>KCETIHVAIVCAGYNASRDVVTLVKSVLFHRRNPLHFHLIADSIAEQILATLFQTWMVPAVRVDFYNADELKSEVSWIPNKHYSGIYGLMKLVLTKTLPANLERVIVLDTDITFATDIAELWAVFHKFKGQQVLGLVENQSDWYLGNLWKNHRPWPALGRGYNTGVILLLLDKLRKMKWEQMWRLTAERELMGMLSTSLADQDIFNAVIKQNPFLVYQLPCFWNVQLSDHTRSEQCYRDVSDLKVIHWNSPKKLRVKNKHVEFFRNLYLTFLEYDGNLLRRELFGCPSEADVNSENLQKQLSELDEDDLCYEFRRERFTVHRTHLYFLHYEYEPAADSTDVTLVAQLSMDRLQMLEAICKHWEGPISLALYLSDAEAQQFLRYAQGSEVLMSRHNVGYHIVYKEGQFYPVNLLRNVAMKHISTPYMFLSDIDFLPMYGLYEYLRKSVIQLDLANTKKAMIVPAFETLRYRLSFPKSKAELLSMLDMGTLFTFRYHVWTKGHAPTNFAKWRTATTPYRVEWEADFEPYVVVRRDCPEYDRRFVGFGWNKVAHIMELDVQEYEFIVLPNAYMIHMPHAPSFDITKFRSNKQYRICLKTLKEEFQQDMSRRYGFAALKYLTA[2x]

Like-acetylglucosaminyltransferase 1 (LARGE1) is a bifunctional glycosyltransferase (GTase) that plays a critical role in maintaining proper muscle function. This enzyme is responsible for a post-translational modification on the extracellular matrix receptor, α-dystroglycan (α-DG), which enables it to interact with proteins containing a laminin-G domain. The polysaccharide which LARGE1 synthesizes, termed matriglycan, is composed of xylose (Xyl) and glucuronic acid (GlcA) subunits in a linear repeating structure of [-3GlcA-β1,3-Xyl-α1-]n. LARGE1 is present in the Golgi as a type II membrane protein, composed of a transmembrane/cytosolic region, a predicted coiled-coil/stem (CC), and domains with xylosyltransferase (Xyl-T) and glucuronyltransferase (GlcA-T) catalytic activities, which are separated by a linker.

While obtaining the single-particle EM data, we also managed to crystallize the LARGE1ΔCC and to collect X-ray diffraction data, extending to 2.6 Å. The crystal of LARGE1 belonged to a C 2 space group, and we found two copies of LARGE1 in the asymmetric unit. For both chains (i.e., A and B), electron density was visible and hence allowed us to model residues 134 to 752. Despite the fact that we have crystallized the LARGE1ΔCC construct, the two chains in the asymmetric unit formed a parallel dimer that resembles the EM map of the LARGE1ecto. Indeed, the crystallographic dimer readily fits into the EM density map of the LARGE1ecto. Inspection of the parallel dimer interface shows an overall buried surface area of 2,589 Å2 (1,350 Å2 on chain ‘A’ and 1239 Å2 on chain ‘B’). In the active site of the Xyl-T domain, we could not detect a clear density that would indicate the presence of a divalent cation. In the electron density map, we observed density for a coordinated ion in the active site of the GlcA-T domain and we therefore modeled a Mn2+ atom, which is an essential metal for the activity of LARGE1. The LARGE1 GlcA-T domain has an extra histidine (His708) that seems to participate in the binding of the Mn2+. Interestingly, the closest Xyl-T and GlcA-T sites in the context of the LARGE1 dimer are located on opposite monomers rather than on a single protomer.> 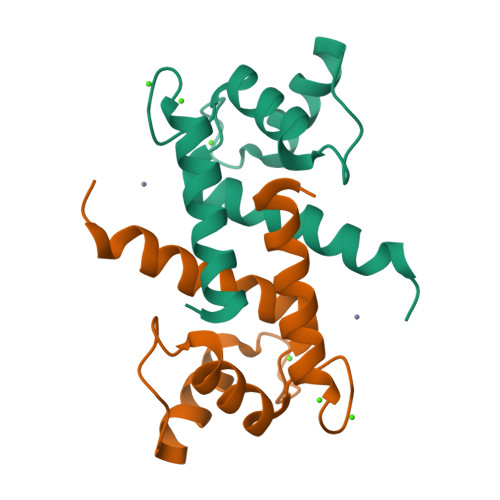MSELEKAMVALIDVFHQYSGREGDKHKLKKSELKELINNELSHFLEEIKEQEVVDKVMETLDNDGDGECDFQEFMAFVAMVTTACHEFFEHE> SNATAFVPALVASGL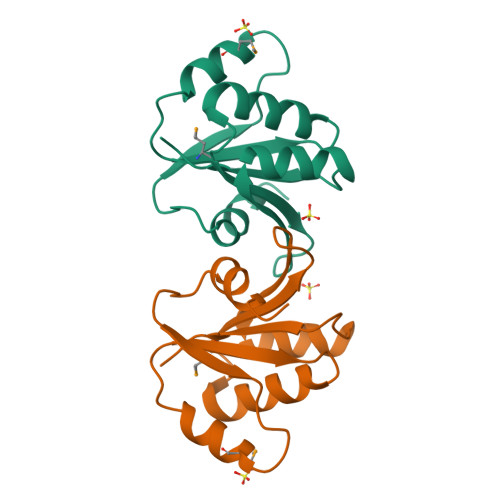PNEKFCFEGFLPQKKGRMTKLKSLVDEHRTMVFYESPHRLLKTLTQFAEYFGPERQVSVSREISKIHEETVRGTLSELIEHFTATDPRGEIVIVLAGIDD> GSAMGSEGLSDVASFATKLKNTLIQYHSIEEDKWRVAKKTKDVTVWRKPSEEFNGYLYKAQGVIDDLVYSIIDHIRPGPSRLDWDSLMTS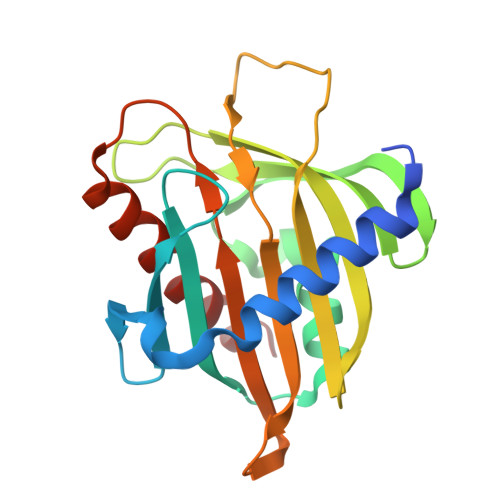LDILENFEENCCVMRYTTAGQGGISPREFVDFSYTVGYKEGLLSCGISLDWDEKRPEFVRGYNHPCGWFCVPLKDNPNQSLLTGYIQTDLRGMIPQSAVDTAMASTLTNFYGDLRKAL> MYEEFRDVITFQSYVEQSNGEGGKTYKWVDEFTAAAHVQPISQEEYYKAQQLQTPIGYNIYTPYDDRIDKKMRVIYRGKIVTFIGDPVDLSGLQEITRIKGKEDGAYV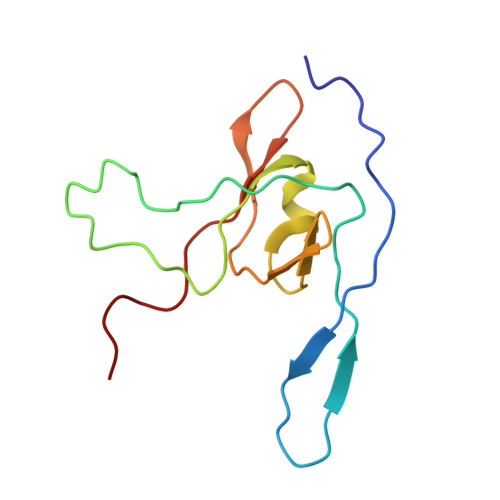G7-oxidanyl-2-oxidanylidene-6-(3,5,5,8,8-pentamethyl-6,7-dihydronaphthalen-2-yl)chromene-3-carboxylic 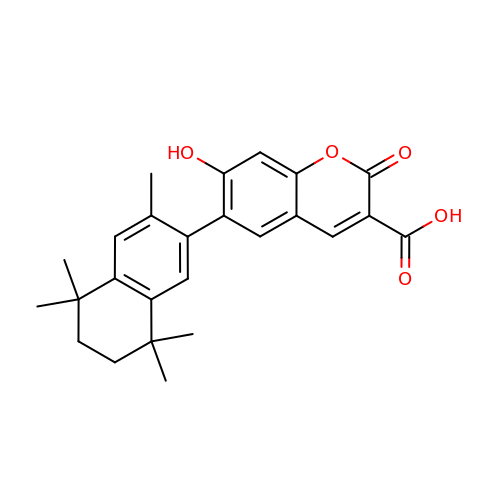acid | C25 H26 O5 | UYPOSIGCFZMVDD-UHFFFAOYSA-N(3-{4-[(2S)-2-(AMINOMETHYL)MORPHOLIN-4-YL]-7H-PYRROLO[2,3-D]PYRIMIDIN-5-YL}PHENYL)METHANOL 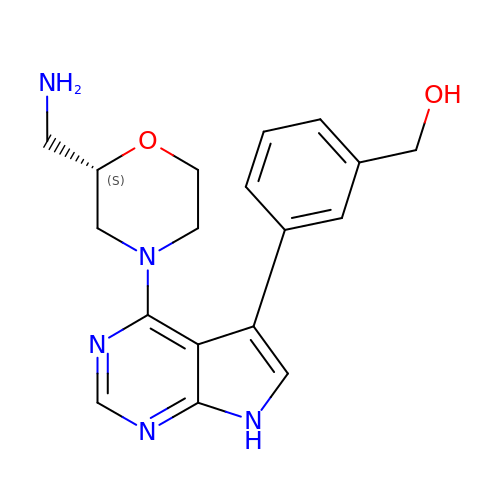| C18 H21 N5 O2 | XYTDDDZEIXYDNO-AWEZNQCLSA-N> SPVGQQYHVEKFSGLRIRKPRVSSSEMERKMNGRKLIRLAQLQNKIATEKLEEEDWVTFGVIVKKITPQSSNNGKTFSIWRLNDLKDLDKYISLFLFGDVHKEHWKTDQGTVIGLLNANPMKPKEGTDEVCLSVDNPQKVLLMGDAVDLGTCKARKKNGDPCTQMVNLNDCEYCQYHVQAQYKKVSSKRADL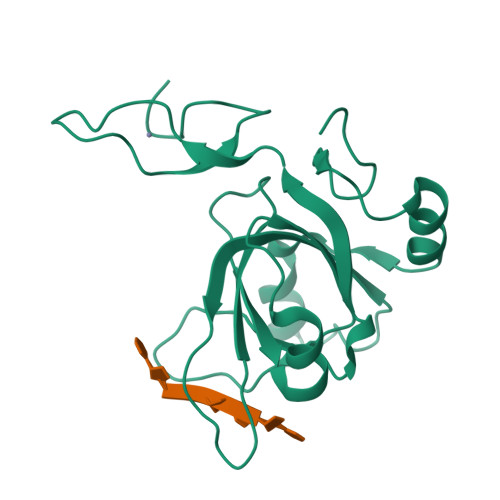QSSYSG>[4x]AESHWCYEVQAESSNYPC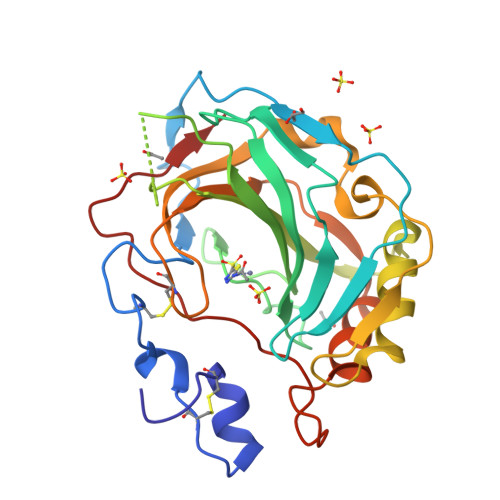LVPVKWGGNCQKDRQSPINIVTTKAKVDKKLGRFFFSGYDKKQTWTVQNNGHSVMMLLENKASISGGGLPAPYQAKQLHLHWSDLPYKGSEHSLDGEHFAMEMHIVHEKEKGTSRNVKEAQDPEDEIAVLAFLVEAGTQVNEGFQPLVEALSNIPKPEMSTTMAESSLLDLLPKEEKLRHYFRYLGSLTTPTCDEKVVWTVFREPIQLHREQILAFSQKLYYDKEQTVSMKDNVRPLQQLGQRTVIKS> MEAVLNELVSVEDLLKFEKKFQSEKAAGSVSK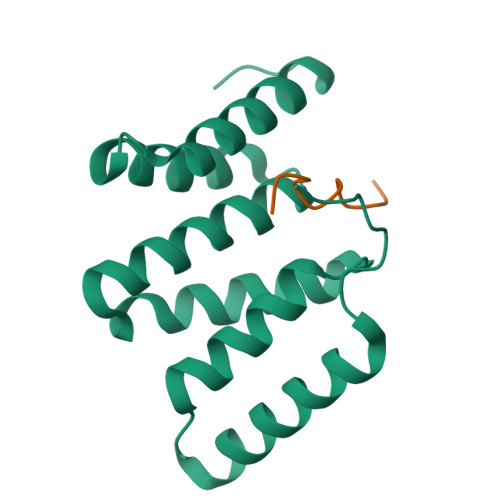STQFEYAWCLVRSKYNDDIRKGIVLLEELLPKGSKEEQRDYVFYLAVGNYRLKEYEKALKYVRGLLQTEPQNNQAKELERLIDKAMKKDGLVG;> SHKHDPLPYPHFLL N-(4-amino-4'-fluoro[1,1'-biphenyl]-3-yl)oxane-4-carboxamide | C18 H19 F N2 O2 | 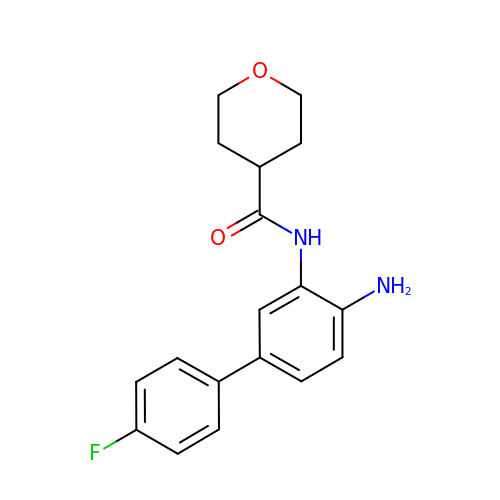ZFCDNONWGMYBHA-UHFFFAOYSA-N Biliverdin IXβ reductase (BLVRB) has emerged as a promising therapeutic target for thrombocytopenia due to its involvement in reactive oxygen species (ROS) mechanisms. In the pathway of heme degradation, BLVRB utilizes NAD(P)H downstream of heme oxygenase(s)-1 (inducible HMOX1) and -2 (constitutive HMOX2) to reduce biliverdin (BV)-IXβ to bilirubin (BR)-IXβ. Consequently, the BV/BR redox cycle, under the control of BLVRB, plays a crucial role in regulating reactive oxygen species (ROS). A large-scale transcriptomic analysis on essential and reactive thrombocytosis cohorts identified biliverdin IXβ reductase (BLVRB) as a regulator of platelet production through MK differentiation by controlling reactive oxygen species (ROS).

To this end, we devised a new chemical scheme to replace the diazenyl bond of olsalazine with an alkene bond, resulting in the creation of olsalkene (OSK). The crystal structures of BLVRB bound to NADP+ and OSK were resolved at a resolution of 1.7 Å. The crystals belong to space group P21212, with each crystal asymmetric unit containing two BLVRB molecules (designated as Mol-A and -B). Notably, a specific region of BLVRB, situated within the vicinity of crystal contacts, exhibits considerable disparity between Mol-A and Mol-B. Particularly, the structures of drug-binding pockets display distinctions between Mol-A and Mol-B. While the OSK-binding pocket structure in Mol-B is influenced by the presence of the second BLVRB molecule due to crystal contacts, the structure of the OSK-binding pocket in Mol-A remains intact in a monomeric state of BLVRB. Consequently, detailed structural analyses of the complex were focused on Mol-A. The binding site of OSK closely associates with the nicotinamide moiety of the NADP+ cofactor, where the xanthene ring of FMN adopts a similar orientation to xanthene-based inhibitors like phloxine B and erythrosine, as evidenced by NMR titration experiments. A primary driving force for the binding of OSK is the ring-stacking interaction between the nicotinamide moiety of NADP+ and OSK, along with hydrophobic interactions involving residues S111, F113, W116, L125, V128, P152, and H153. Additionally, favorable interactions are facilitated by positively charged residues R78, K120, R124, R170, and K178. Notably, OSK displaces the sidechain of W116 (as observed in the FMN complex) and shifts it toward the binding pocket by approximately 2.5 Å. OSK exhibited high affinity and specific binding to the substrate binding pocket of BLVRB with a KD of 0.140 µM, akin to the previously studied OSA.

>[2x]MAVKKIAIFGATGQTGLTTLAQAVQAGYEVTVLVRDSSRLPSEGPRPAHVVVGDVLQAADVDKTVAGQDAVIVLLGTRNDLSPTTVMSEGARNIVAAMKAHGVDKVVACTSAFLLWDPTKVPPRLQAVTDDHIRMHKVLRESGLKYVAVMPPHIGDQPLTGAYTVTLDGRGPSRVISKHDLGHFMLRCLTTDEYDGHSTYPSHQYQ> DVDKNDLKKKSDIDSSKLFNLTSYYTDITWQLDESNKISTDQLLNNTIILKDIDISVLKTSSLKVEFNSSDLANQFKGKNIDIYGLYYGNKCVGLTEEKTSCLYGGVTIYDGNQLDEERVIGVNVFKDGIQQEGFVIKTKKAKVTVQELDTKVRFKLENLYKIYNKDTGNIQKGCIFFHSNNHQNQSFYYDLYNIKGSVGAEFFQFYSDNRTVSSSNYHIDVFLYKD

Superantigens (SAgs) are the critical virulence factors of Staphylococcus aureus. SAgs can cross-bridge the major histocompatibility complex class II (MHC II) with T cell receptor (TCR) molecules to stimulate a massive proliferation of T cells (~20–30%) in a relatively nonspecific manner. The multiple X-ray structures of staphylococcal SAgs revealed that the protein is composed of an N-terminal oligonucleotide-binding (OB) fold and a C-terminal β-grasp domain. SEN belongs to the group III SAg as revealed by multiple amino acid sequence alignment.

The structure of SEN was solved by molecular replacement, and the final model was refined at 1.8 Å resolution (Rwork = 0.171, Rfree = 0.201). There is one monomer per asymmetric unit. Overall, SEN is a compact molecule and shows the classic two-domain architecture of SAg proteins. The N-terminal OB-fold domain (residues 52–137) consists of five-stranded β-barrel (β1, β2, β3, β4, β5a, and β5b) and two 310 helices (310 1 and 310 2). The C-terminal β-grasp domain of SEN consists of anti-paralleled β-strands (β6–β12) and α-helices (α4 and α5). Superposition of SEN and other SAg structures revealed that in the SEN structure, an asparagine (Asn44) is situated in a nearly identical position to that in the other SAgs. However, the aromatic pair is not present in the equivalent position in SEN. The corresponding amino acids in the position are Gly113 and Asn114. These amino acid variations might confer TRBV specificity to SEN. The ion-coordinating amino acids and their stabilizing amino acids are present in the structure of SEN.>[2x]MDMLWHKLPKSIYFRRGSLPIALDEVITDGHKRALIVTDRFLFNNGYADQITSVLKAAGVETEVFFEVEADPTLSIVRKGAELANSFKPDVIIALGGGSPMDAAKIMWVMYEHPE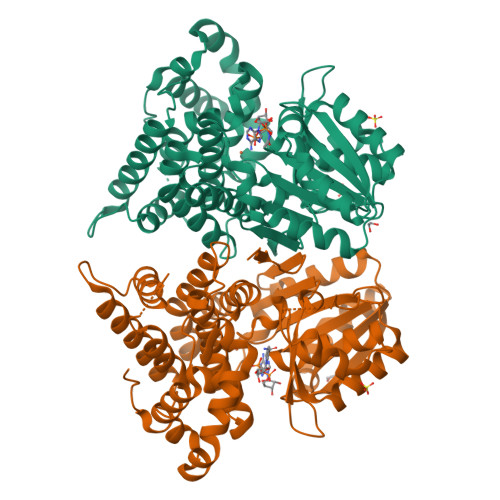THFEELALRFMDIRKRIYKFPKMGVKAKMIAVTTTSGTGSEVTPFAVVTDDATGQKYPLADYALTPDMAIVDANLVMDMPKSLCAFGGLDAVTHAMEAYVSVLASEFSDGQALQALKLLKEYLPASYHEGSKNPVARERVHSAATIAGIAFANAFLGVCHSMAHKLGSQFHIPHGLANALLICNVIRYNANDNPTKQTAFSQYDRPQARRRYAEIADHLGLSAPGDRTAAKIEKLLAWLETLKAELGIPKSIREAGVQEADFLANVDKLSEDAFDDQCTGANPRYPLISELKQILLDTYYGRDYVEGETAAKKEAAPAKAEKKAKKSAPWGAGGLEVLFQ> MSSVLKAFERFTIEQELQDRGEEGSIPPETLKSAVKVFVINTPNPTTRYQMLNFCLRIICSQNARASHRVGALITLFSLPSAGMQNHIRLADRSPEAQIERCEIDGFEPGTYRLIPNARANLTANEIAAYALLADDLPPTINNGTPYVHADVEGQPCDEIEQFLDRCYSVLIQAWVMVCKCMTAYDQPAGSADRRFAKYQQQGRLEARYMLQPEAQRLIQTAIRKSLVVRQYLTFELQLARRQGLLSNRYYAMVGDIGKYIENSGLTAFFLTLKYALGTKWSPLSLAAFTGELTKLRSLMMLYRDIGEQARYLALLEAPQIMDFAPGGYPLIFSYAMGVGTVLDAQMRNYTYARPFLNGYYFQIGVETARRQQGTVDNRVADDLGLTPEQRT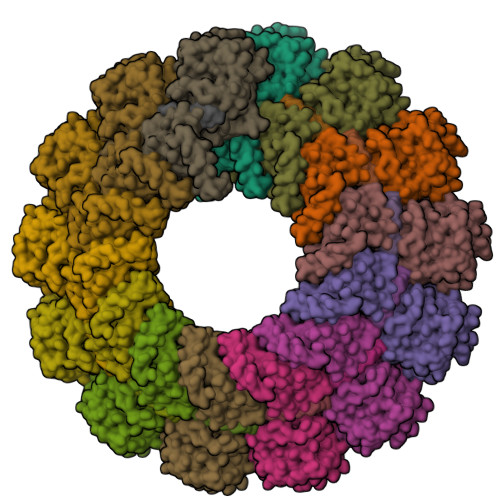EVTQLVDRLARGRGAGIPGGPVNPFVPPVQQQQPAAVYADIPALEESDDDGDEDGGAGFQNGVQVPAVRQGGQTDFRAQPLQDPIQAQLFMPLYPQVSNIPSNQNHQINRIGGLENQDLLRYNENGDSQQDARGEHGNTFPNNPNQNAQLQVGDWDE> RQIRLIGQSCTAPKIHMDCSNLTALATSKPRALSCQTLAAGYYHTECVSGCVCPDGLMDDGRGGCVVEKECPCVHNNDLYSSGAKIKVDCNTCTCKRGRWVCTQAVCHGTCSIYGSGHYITFDGKYYDFDGHCSYVAVQDYCGQNSSLGSFSIITENVPCGTTGVTCSKAIKIFMGRTELKLEDKHRVVIQRDEGHHVAYTTREVGQYLVVESSTGIIVIWDKRTTVFIKLAPSYKGTVCGLCGNFDHRSNNDFTTRDHMVVSSELDFGNSWKEAPTCPDVSTNPEPCSLNPHRRSWAEKQCSILKSSVFSICHSKVDPKPFYEACVHDS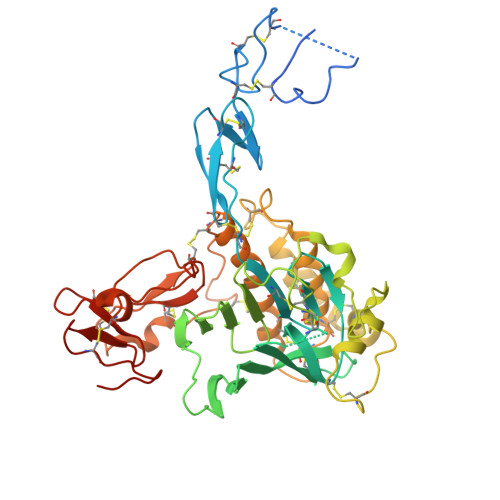CSCDTGGDCECFCSAVASYAQECTKEGACVFWRTPDLCPIFCDYYNPPHECEWHYEPCGNRSFETCRTINGIHSNISVSYLEGCYPRCPKDRPIYEEDLKKCVTADKCGCYVEDTHYP>GASEPSGPPTDLWVESRGPFTILVRWKAPPKEYWHGKLKGYYVGYKMEGSPQPYSFKTVEAMNVNITHEYLLNSLKKSTKYSIVVKAYNAAGTGPASQELIVKTLDGVLPRPPSVSLLSASDSTISVKWGHTISRDEPVTGYTLHYRKKVGHWLHVPLLASDQTRYTLTGLDSDTTYNVYVTANNRYGRGDPSGILSVRTGD[7x]

Recently, a shortened Dscam (sDscam) gene family with tandemly arrayed 5′ cassettes in Chelicerata species has been identified, which encodes ∼50–100 isoforms. Chelicerata sDscams could be classified into two subfamilies, sDscamα and sDscamβ, containing one and two variable Ig domains, respectively. Crystal structures and cell aggregation assays demonstrated that both α and β subfamilies of sDscam used Ig1 for the isoform-specific trans recognition in a hand-in-hand manner. Furthermore, the cis interactions were established by the three FNIII domains of sDscam, which assemble into a cross fold with a kink between FNIII2 and FNIII3.

Thus, this kink conformation may reflect a physiological geometric assembly. The inter-domain interface of the kink contains a salt bridge formed by R404 and D578, and the hydrophobic interaction mediated by L492 and L496. The cis interactions are mediated by the FNIII domains that are constant within the sDscam subfamilies.>AMKNWKTSAESILTTGPVVPVIVVKKLEHAVPMAKALVAGGVRVLNVTLRTECAVDAIRAIAKEVPEAIVGAGTVLNPQQLAEVTEAGAQFAISPGLTEPLLKAATEGTIPLIPGISTVSELMLGMDYG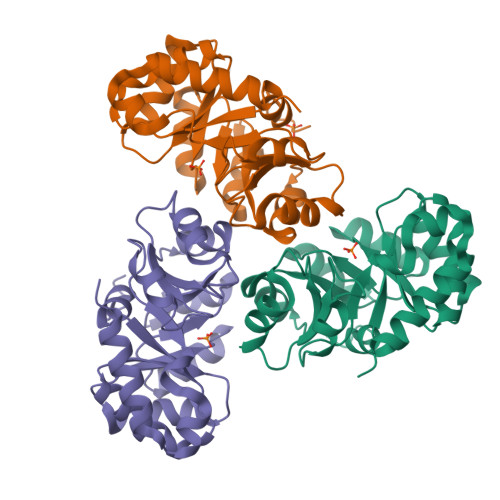LKEFKFFPAEANGGVKALQAIAGPFSQVRFCPTGGISPANYRDYLALKSVLCIGGSWLVPADALEAGDYDRITKLAREAVEGAKL[3x]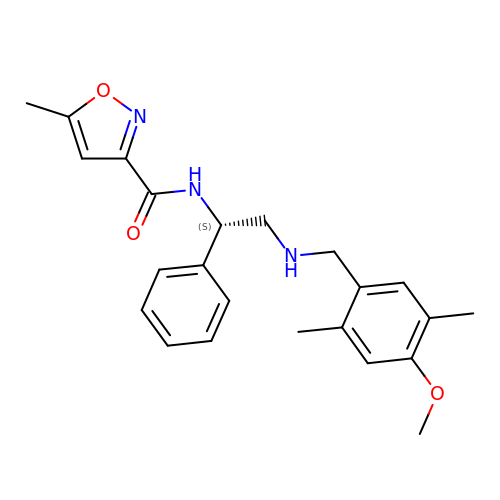~{N}-[(1~{S})-2-[(4-methoxy-2,5-dimethyl-phenyl)methylamino]-1-phenyl-ethyl]-5-methyl-1,2-oxazole-3-carboxamide | C23 H27 N3 O3 | JWARISOWNKYPRB-OAQYLSRUSA-N> MGMRVLVTTWGNPFQWEPI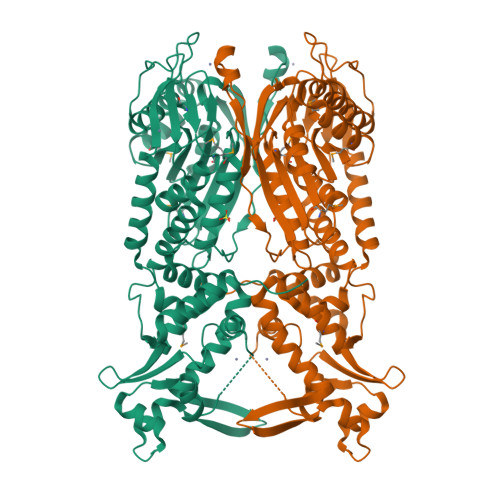TYEYRGIKVKSRNTLPILVKTLEPERILILVADTMANYYDSGKNKPEIEEKSFSSYSEVVEDTKERILWHIKEEVIEELREEDPELAKKIENMLKDERITIEVLPGVGVFGNITVEGEMLDFYYYATYKLAEWLPVQNNLEVYLDLTHGINFMPTFTYRALRNLLGLLAYLYNVKFEIVNSEPYPLGVSQEIREDTILHIREIGEGVVRPRPQYSPVEGKLYWNAFISSVANGFPLVFASFYPNIRDVEDYLNKKLEEFLVGIEVGEREDGKPYVKREKALDRSFKNASKLYYALRVFNTKFQNYPKKEVPIEEIMEISKIFESLPRIGIILERQVEWLRNLVYGRLWYENGEQKIKKGLLEIIKDKKDKRKEAEALKKGKTISLAEAAKLTRIFSPSGERIETIESPNVVRNFIAHSGFEYNIVYVKYDRLSDRLYFFYKDKEKAANLAYEALLYRGEKE>MDQTYSLESFLNHVQKRDPNQTEFAQAVREVMTTLWPFLEQNPKYRQMSLLERLVEPERVIQFRVVWVDDRNQIQVNRAWRVQFSSAIGPYKGGMRFHPSVNLSILKFLGFEQTFKNALTTLPMGGGKGGSDFDPKGKSEGEVMRFCQALMTELYRHLGADTDVPAGDIGVGGREVGFMAGMMKKLSNNTACVFTGKGLSFGGSLIRPEATGYGLVYFTEAMLKRHGMGFEGMRVSVSGSGNVAQYAIEKAMEFGARVITASDSSGTVVDESGFTKEKLARLIEIKASRDGRVADYAKEFGLVYLEGQQPWSLPVDIALPCATQNELDVDAAHQLIANGVKAVAEGANMPTTIEATELFQQAGVLFAPGKAANAGGVATSGLEMAQNAARLGWKAEKVDARLHHIMLDIHHACVEHGGEGEQTNYVQGANIAGFVKVADAMLAQGVI[6x]

In all, we determined 23 structures, four of them not deposited in the protein data bank. These novel structures represent enzymes involved in stress response, specifically methylglyoxal reductase (YghZ), as well as three enzymes important in core metabolic functions, phosphoglucose isomerase (pGI), 6-phospho-beta-glucosidase (BglA), and glutamate dehydrogenase (GDH). All the proteins are oligomeric (YghZ, pGI, BglA, GDH) and belong to three different fold families. YghZ and BglA have a classic TIM barrel structure, pGI adopts an alpha/beta fold, and GDH possesses a core Rossmann fold found in many nucleotide binding proteins. Based on these experiments, we demonstrate successful structural characterization of multiple proteins using only microgram quantities of purified material.

Glutamate dehydrogenase (GDH), catalyzes the reversible oxidative deamination of glutamate to α-ketoglutarate and ammonia, using either NAD+ or NADP+ as a cofactor. The reverse reaction generates glutamate and the reduced cofactor NADH or NADPH, thus GDH has a pivotal role between carbon and nitrogen metabolism, particularly in plants and bacteria. The majority of characterized glutamate dehydrogenases are homo-oligomers, consisting of between two to six subunits, with dimers being the most frequent. GDH from E. coli crystallized as a hexamer, consistent with biochemical observations, and contains two domains – a larger C-terminal Rossmann fold containing domain and a second N-terminal helical capping domain. The putative active site is located in a cleft between the two domains.5,5'-butane-1,4-diylbis(1,3,4-thiadiazol-2-amine) | C8 H12 N6 S2 | 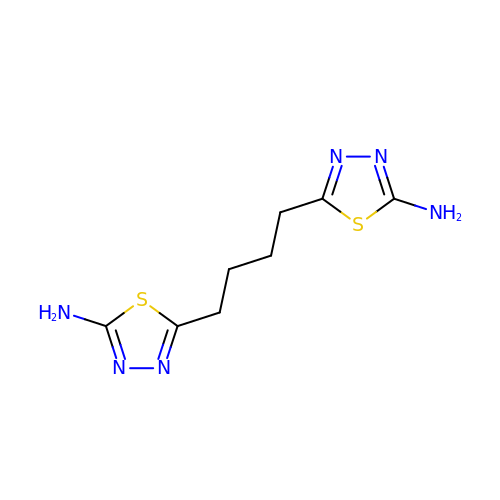FXLSMCSUYSZCFA-UHFFFAOYSA-N>[4x]DQGCAINFGKRELKCGDGIFIFRDSDDWLNKYSYYPEDPVKLAS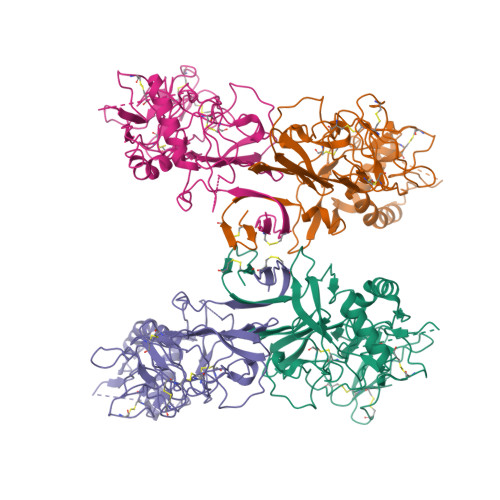IVKASFEEGKCGLNSVDSLEHEMWRSRADEINAIFEENEVDISVVVQDPKNVYQRGTHPFSRIRDGLQYGWKTWGKNLVFSPGRKNGSFIIDGKSRKECPFSNRVWNSFQIEEFGTGVFTTRVYMDAVFEYTIDCDGSILGAAVNGKKSAHGSPTFWMGSHEVNGTWMIHTLEALDYKECEWPLTHTIGTSVEESEMFMPRSIGGPVSSHNHIPGYKVQTNGPWMQVPLEVKREACPGTSVIIDGNCDGRGKSTRSTTDSGKVIPEWCCRSCTMPPVSFHGSDGCWYPMEIRPRKTHESHLVRSWVTAHHHHHH>[3x]AHCIGITDRDFIEGVHGGTWVSATLEQDKCVTVMAPDKPSLDISLETVAIDRPAEVRKVCYNAVLTHVKINDKCPSTGEAHLAEENEGDNACKRTYSD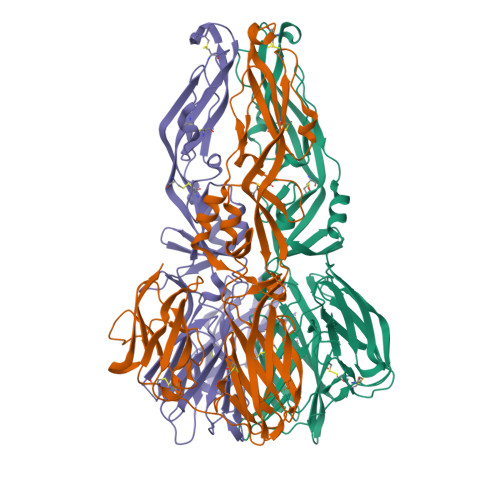RGWGNGCGLFGKGSIVACAKFTCAKSMSLFEVDQTKIQYVIRAQLHVGAKQENWNTDIKTLKFDALSGSQEVEFIGYGKATLECQVQTAVDFGNSYIAEMETESWIVDRQWAQDLTLPWQSGSGGVWREMHHLVEFEPPHAATIRVLALGNQEGSLKTALTGAMRVTKDTNDNNLYKLHGGHVSCRVKLSALTLKGTSYKICTDKMFFVKNPTDTGHGTVVMQVKVSKGAPCRIPVIVADDLTAAINKGILVTVNPIASTNDDEVLIEVNPPFGDSYIIVGRGDSRLTYQWHKEGSS> MSTPDNHGKKAPQFAAFKPLTTVQNANDCCCDGACSSSPTLSENVSGTRYSWKVSGMDCAACARKVENAVRQLAGVNQVQVLFATEKLVVDADNDIRAQVESAVQKAGYSLRDEQAADEPQASRLKENLPLITLIVMMAISWGLEQFNHPFGQLAFIATTLVGLYPIARQALRLIKSGSYFAIETLMSVAAIGALFIGATAEAAMVLLLFLIGERLEGWAASRARQGVSALMALKPETATRLRNGEREEVAINSLRPGDVIEVAAGGRLPADGKLLSPFASFDESALTGESIPVERATGDKVPAGATSVDRLVTLEVLSEPGASAIDRILKLIE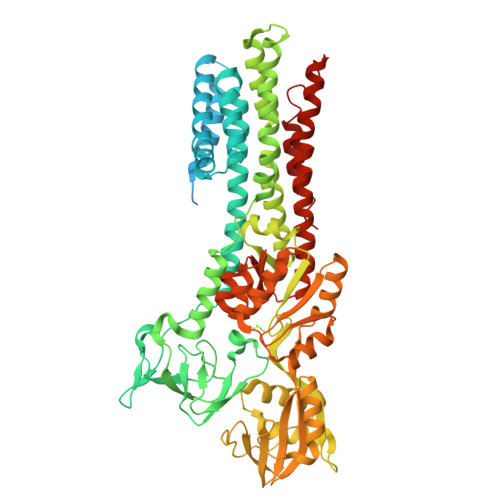EAEERRAPIERFIDRFSRIYTPAIMAVALLVTLVPPLLFAASWQEWIYKGLTLLLIGCPCALVISTPAAITSGLAAAARRGALIKGGAALEQLGRVTQVAFDKTGTLTVGKPRVTAIHPATGISESELLTLAAAVEQGATHPLAQAIVREAQVAELAIPTAESQRALVGSGIEAQVNGERVLICAAGKHPADAFAGLINELESAGQTVVLVVRNDDVLGIIALQDTLRADAATAISELNALGVKGVILTGDNPRAAAAIAGELGLEFKAGLLPEDKVKAVTKLNQHAPLAMVGDGINDAPAMKAAAIGIAMGSGTDVALETADAALTHNHLRGLVQMIELARATHANIRQNITIALGLKGIFLVTTLLGMTGLWLAVLADTGATVLVTANALRLLRRR> SGTGLGEVDVDTYLSNLQTKTTLSMIADGLERSARDFDAFLEENVTLEWEAQRKRIYQH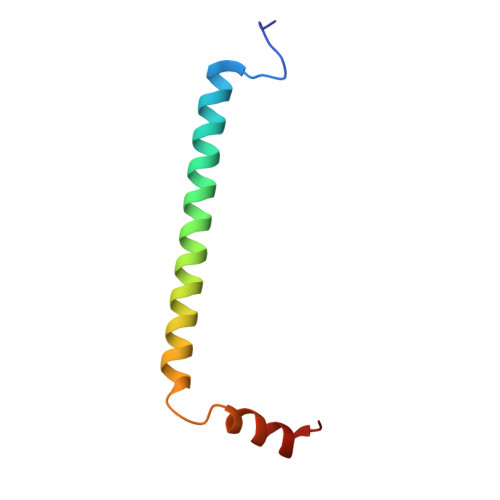FGIK The ferrous iron transport (Feo) system is the primary prokaryotic Fe2+ import machinery, and two constituent proteins (FeoA and FeoB) are conserved across most bacterial species. The function of FeoA is unknown, but we do know that FeoA is an ≈8-kDa, cytoplasmic β-barrel protein comprising an Src homology 3 (SH3)–like fold, which is commonly involved in protein–protein interactions. Interestingly, in some pathogens such as Porphyromonas gingivalis (the causative agent of gingivitis) and Bacteroides fragilis (a commensal organism implicated in drug-resistant peritoneal infections), the feo operon is predicted to encode a single FeoAB fusion protein in which FeoA is naturally tethered to the soluble G-protein domain of FeoB. Herein, we provide the first biochemical and biophysical characterization of the soluble domain of the B. fragilis FeoAB fusion protein (BfNFeoAB).

However, after ≈11 months of equilibration, crystals were obtained in ammonium sulfate and dipotassium phosphate that were further optimized by grid screening. Despite the age of the crystals, diffraction was routinely observed to <2 Å resolution, with our best datasets extending to 1.50 Å. Initial refinement revealed the presence of two molecules of only the FeoA domain (BfFeoA) in the asymmetric unit (ASU). After iterative rounds of rebuilding and refinement, our BfFeoA model converged with Rw = 0.192 and Rf = 0.236. The β-barrel is composed of five β-strands, while two α-helices make up the clamp region of BfFeoA, which comprises a series of hydrophobic residues (Phe23, Ile27, Met30, Ile59, and Leu61) that we have hypothesized to be important for mediating FeoA–NFeoB interactions. An additional 310-helix at the beginning of the N-terminus contacts both the final α-helix and β-strand that feed out of and into the hydrophobic clamp, respectively. Residues comprising both the linker region between FeoA and NFeoB are completely absent from the structure, likely a result of proteolytic degradation in the crystallization drop over time. While sequence analysis of the FeoA polypeptide does not suggest this is a common proteolytic site, the new C-terminus created after proteolysis is unambiguously present in the electron density. The overall structure of BfFeoA is similar to other FeoA proteins that have been determined by NMR or X-ray crystallography, including the hydrophobic cleft putatively involved in protein–protein interactions, suggesting that the FeoA domain in an FeoAB fusion may function similarly to stand-alone FeoA proteins.

>MRLSELKTGEKGVIVKVLGHGGFRKRIVEMGFIKGKTVEVLLNAPLKDPIKYKIMGYEISLRRQEADMIEIISEQE[2x]>MGFKEYPAGEPVTMNEMELAAVYLQPIDMEPRGMGLPAAKADVHLEADIHAVEGNKNGFGAGEWIPYLTISYTLVNNDTGEKQEGTFMPIVASDGPHYGANIKMMGVGNYKVTYHIEPPSKAGMHRHTDSETGVGRW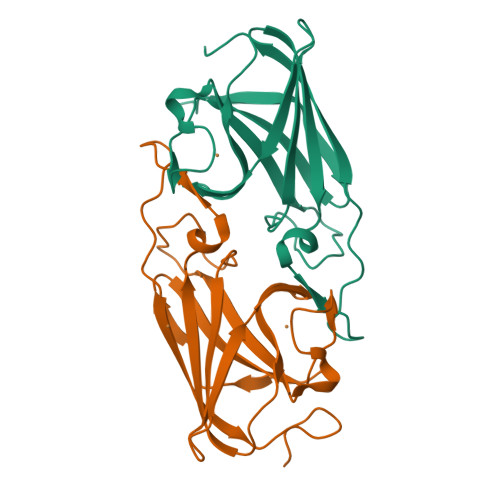WKPFDVSYEFKYVGLNSSGLVPR[2x]>GHMAKQYDSVECPFCDEVSKYEKLAKIGQGTFGEVFKARHRKTGQKVALKKVLMENEKEGFPITALREIKILQLLKHENVVNLIEICRTKASPYNRCKGSIYLVFDFCEHDLAGLLSNVLVKFTLSEIKRVMQMLLNGLYYIHRNKILHRDMKAANVLITRDGVLKLADFGLARAFSLAKNSQPNRYTNRVVTLWYRPPELLLGERDYGPPIDLWGAGCIMAEMWTRSPIMQGNTEQHQLALISQLCGSITPEVWPNVDNYELYEKLELVKGQKRKVKDRLKAYVRDPYALDLIDKLLVLDPAQRIDSDDALNHDFFWSDPMPSDLKGMLST[3x];>MEGERKNNNKRWYFTREQLENSPSRRFGVDPDKELSYRQQAANLLQDMGQRLNVSQLTINTAIVYMHRFYMIQSFTQFPGNSVAPAALFLAAKVEEQPKKLEHVIKVAHTCLHPQESLPDTRSEAYLQQVQDLVILESIILQTLGFELTIDHPHTHVVKCTQLVRASKDLAQTSYFMATNSLHLTTFSLQYTPPVVAC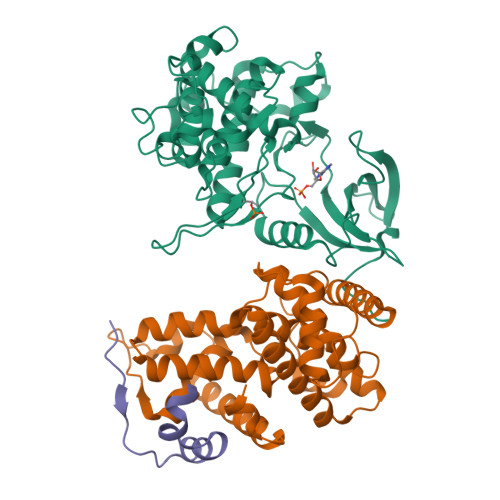VCIHLACKWSNWEIPVSTDGKHWWEYVDATVTLELLDELTHEFLQILEKTPNRLKRIWNWRACEAA[3x];>SNANREDRNVLRMKERERRNQEIQQGEDAFPPSSPLFAEPYKVTSKEDKLSSRIQSMLGNYDEMKDFIGDRSIPK[3x]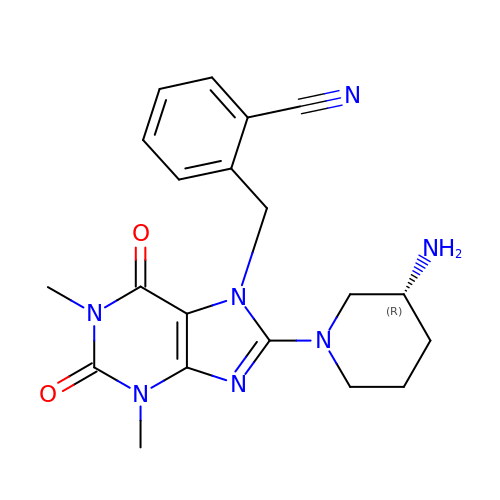2-({8-[(3R)-3-AMINOPIPERIDIN-1-YL]-1,3-DIMETHYL-2,6-DIOXO-1,2,3,6-TETRAHYDRO-7H-PURIN-7-YL}METHYL)BENZONITRILE | C20 H23 N7 O2 | XJNKUWDMCBZMTG-OAHLLOKOSA-N>MPLSPILRQILQQLAAQLQFRPDMDVKTVREQFEKSSLILVKMANEPIHRVEDITIPGRGGPI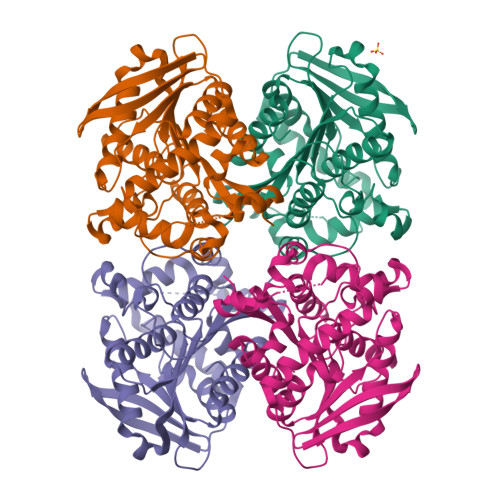RARVYRPRDGERLPAVVYYHGGGFVLGSVETHDHVCRRLANLSGAVVVSVDYRLAPEHKFPAAVEDAYDAAKWVADNYDKLGVDNGKIAVAGDSAGGNLAAVTAIMARDRGESFVKYQVLIYPAVNLTGSPTVSRVEYSGPEYVILTADLMAWFGRQYFSKPQDALSPYASPIFADLSNLPPALVITAEYDPLRDEGELYAHLLKTRGVRAVAVRYNGVIHGFVNFYPILEEGREAVSQIAASIKSMAVA[4x]>[6x]MHHHHHHEEQGHSEMEIIPSESHPHIQLLKSNRELLVTHIRNTQCLVDNLLKNDYFSAEDAEIVCACPTQPDK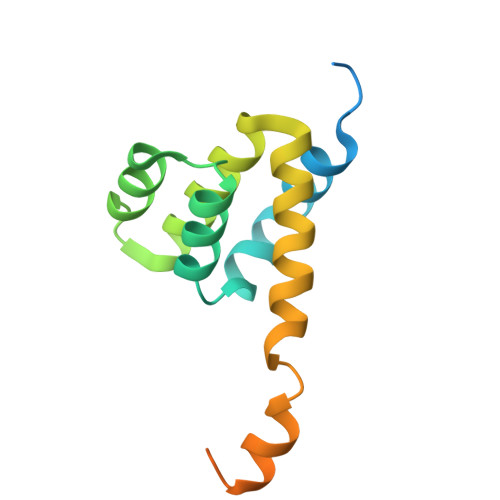VRKILDLVQSKGEEVSEFFLYLLQQLADAYVDLRPWLLEIGFSPSLLTQSKVVVNTDPVSRYTQQLRHHLG>[6x]AMGNKLFNIAQRILDTNSVLLTERGDYIVWINNSWKFNSEEPLITKLILSIRHQLPKEYSSELLCPRKRKTVEANIRDMLVDSVETDTYPDKLPFKNGVLDLVDGMFYSGDDAKKYTCTVSTGFKFDDTKFVEDSPEMEELMNIINDIQPLTDENKKNRELYEKTLSSCLCGATKGCLTFFFGETATGKSTTKRLLKSAIGDLFVETGQTILTDVLDKGPNPFIANMHLKRSVFCSELPDFACSGSKKIRSDNIKKLTEPCVIGRPCFSNKINNRNHATIIIDTNYKPVFDRIDNALMRRIAVVRFRTHFSQPSGREAAENNDAYDKVKLLDEGLDGKIQNNRYRFAFLYLLVKWYKKYHVPIMKLYPTPEEIPDFAFYLKIGTLLVSSSVKHIPLMTDLSKKGYILYDNVVTLPLTTFQQKISKYFNSRLFGHDIESFINRHKKFANVSDEYLQYIFIEDISSP

The helicase-primase D5, composed of six identical 90 kDa subunits, is required for DNA replication. As the ribonucleotide hydrolase activity of D5323–785 had also been indistinguishable from D5fl, we used the D5323–785 construct for high-resolution work, assisted by an Alphafold2 prediction, which yielded a structure of D5 with a high reliability index and allowed us to assign five domains: the primase domain and a distinct Zn-binding (or Cys-cluster) domain in the N-terminal polypeptide not present in D5323–785 used for cryo-EM reconstruction, a collar domain, an AAA+ helicase domain, and a C-terminal domain. The sample used for the cryo-EM data collection contained a roughly equimolar complex of D5323–785 hexamer with a dsDNA 30-mer obtained by mixing.

Cryo-EM of D5323–785 yielded a variety of projections that generated an electron density map with a nominal resolution of 4.1 Å based on the half-set Fourier shell correlation when six-fold symmetry was inferred. The electron density showed an organization in three domains, which could be fitted with the Alphafold2 models of the corresponding domains. The density corresponding to the collar domain is defined best with estimated local resolutions of 3.9 to 4.5 Å (a sample of the density is shown in Figure 3b). The electron density of the C-terminal domain was also weaker, requiring a lower contour level. Due to the low resolution of the C-terminal domain, the final model stayed as close as possible to the Alphafold2 model. The refined structure of D5323–785 conserves largely the geometrical quality of the initial Alphafold2 model (third column), which it matches very well with an rms deviation of 1.3 Å for all atoms. The hexamer shows a central channel with a minimal diameter of about 16 Å at three points of constriction: the level of the basic cluster in the collar domain (21 Å), the β-hairpin loop (16 Å), and the DNA binding loop in the AAA+ helicase domain (18 Å). The channel would just be sufficiently wide for the passage of dsDNA. In our structure, any additional electron density, which could be interpreted as nucleotide, was missing so that no information about the nucleotide-binding site could be obtained.>[2x]GSKEGEYIKLKVIGQDSSEIHFKVKMTTHL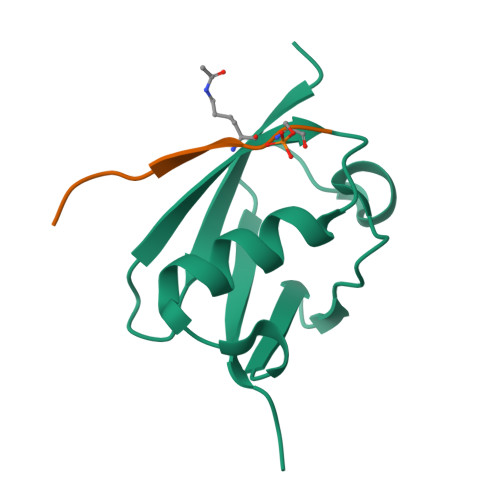KKLKESYAQRQGVPMNSLRFLFEGQRIADNHTPKELGMEEEDVIEVYQEQTGG;>GSGEAEERIIVLSDSDY[2x]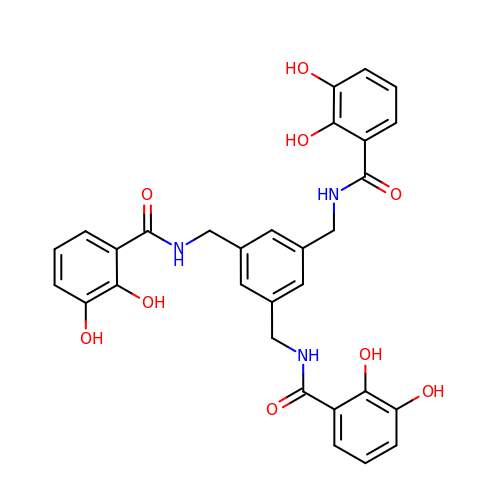N,N',N''-[BENZENE-1,3,5-TRIYLTRIS(METHYLENE)]TRIS(2,3-DIHYDROXYBENZAMIDE) | C30 H27 N3 O9 | GCTFIRZGPIUOAK-UHFFFAOYSA-N The phosphorolytic exoribonuclease polynucleotide phosphorylase (PNPase; EC 2.7.7.8) is encoded in the genomes of bacteria and eukaryotes, and in those domains of life the ribonuclease plays multifaceted roles in regulation and environmental response. While the C-terminal RNase PH-like domain catalyses phosphorolytic attack of RNA, the N-terminal domain has lost this capacity; instead, it contributes to the ring-like quaternary structure of the trimeric PNPase assembly. Two recurrent structural motifs that are found in many RNA-binding proteins, the S1 and K-homology (KH) domains, are appended at the C-terminus of PNPase. The PNPase studied here is from the bacterium Caulobacter crescentus, which has been established as a model system to investigate cell cycle progression, because populations can be readily prepared that are synchronized in the cell cycle.

Caulobacter crescentus PNPase was co-crystallized with a short peptide corresponding to its recognition motif from RNase E in two different space groups (P63 and R3). The asymmetric unit of the rhombohedral crystals contains three PNPase protomers, while the hexagonal crystal form contains a single protomer. Although no electron density was apparent for the KH and S1 domains of PNPase in the rhombohedral crystal form, clear density was present for these domains in the hexagonal crystal. The KH and S1 domains were manually built into this density using as guides the NMR model of the isolated PNPase S1 domain and the X-ray structure of a KH domain from human vigillin. The three KH domains are positioned over the entrance to the catalytic core like an umbrella, with the RNA-binding GSGG loops (residues 572–575) forming a secondary entrance aperture. The S1 domains adopt a splayed conformation, and the conformation is constrained by the crystal packing. We suggest that the S1 domains are flexibly tethered to the KH domains, and that they potentially could manoeuvre to capture RNA substrates as part of a molecular fly-casting mechanism. The RNA-binding surfaces of the S1 domains face the molecular threefold axis at the centre of the PNPase trimer, and it is envisaged that S1 domains could clamp down in concert on RNA targets. Crystals of RNA-free PNPase with recognition peptide (KPRRGWWR) revealed clear density for the peptide in both the hexagonal and rhombohedral crystal forms of PNPase. In the hexagonal crystal form, the GWW peptide additionally forms crystal packing contacts with the S1 domain of a neighbouring molecule.

> MGSSHHHHHHSQSPMFDIKRKTIEWGGKTLVLETGRIARQADGAVLATMGETVVLATAVFAKSQKPGQDFFPLTVNYQEKTFAAGKIPGGFFKREGRPSEKETLVSRLIDRPIRPLFVKGFKNEVQVVVTVLQHDLENDPDILGMVAASAALCLSGAPFMGPIGAARVGWVDGAYVLNPTLDEMKESKMDLVVAGTADAVMMVESEIQELSEEIVLGGVNFAHQQMQAVIDAIIDLAEHAAKEPFAFEPEDTDAIKAKMKDLVGADIAAAYKIQKKQDRYEAVGAAKKKAIAALGLSDENPTGYDPLKLGAIFKELEADVVRRGILDTGLRIDGRDVKTVRPILGEVGILPRTHGSALFTRGETQAIVVATLGTGDDEQFIDALEGTYKESFLLHYNFPPYSVGETGRMGSPGRREIGHGKLAWRALRPMLPTKEDFPYTIRLVSEITESNGSSSMATVCGSSLAMMDAGVPLVRPVSGIAMGLILEQDGFAVLSDILGDEDHLGDMDFKVAGTSEGLTSLQMDIKIAGITPAIMEQALAQAKEGRAHILGEMNKAMDAPRADVGDFAPKIETINIPTDKIREVIGSGGKVIREIVATTGAKVDINDDGVVKVSASDGAKIKAAIDWIKSITDEAEIGKIYDGKVVKVVDFGAFVNFFGAKDGLVHVSQISNERVAKPSDVLKEGQMVKVKLLGFDDRGKTKLSMKVVDQETGEDLSKKEAAAEEA;> TAPPEKPRRGWWRR> VKDTYTDRLDDWNGIIAGNQYYDSKNDQMAKLNQELEGKVADSLSSISSQADRIYLWEKFSNYKTSANLTATYRKLEEMAKQVTNPSSRYYQDETVVRTVRDSMEWMHKHVYNSEKSIVGNWWDYEIGTPRAINNTLSLMKEYFSDEEIKKYTDVIEKFVPDPEHFRKTTDNPFKALGGNLVDMGRVKVIAGLLRKDDQEISSTIRSIEQVFKLVDQGEGFYQDGSYIDHTNVAYTGAFGNVLIDGLSQLLPVIQKTKNPIDKDKMQTMYHWIDKSFAPLLVNGELMDMSRGRSISRANSEGHVAAVEVLRGIHRIADMSEGETKQRLQSLVKTIVQSDSYYDVFKNLKTYKDISLMQSLLSDAGVASVPRTSYLSAFNKMDKTAMYNAEKGFGFGLSLFSSRTLNYEHMNKENKRGWYTSDGMFYLYNGDLSHYSDGYWPTVNPYKMPGTTETDAKR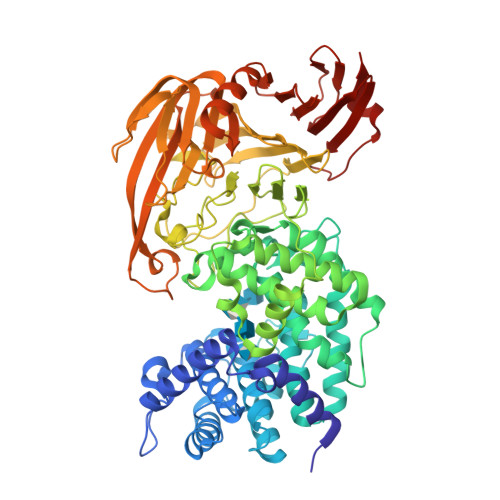ADSDTGKVLPSAFVGTSKLDDANATATMDFTNWNQTLTAHKSWFMLKDKIAFLGSNIQNTSTDTAATTIDQRKLESSNPYKVYVNDKEASLTEQEKDYPETQSVFLESSDSKKNIGYFFFKKSSISMSKALQKGAWKDINEGQSDKEVENEFLTISQAHKQNGDSYGYMLIPNVDRATFNQMIKELESSLIENNETLQSVYDAKQGVWGIVKYDDSVSTISNQFQVLKRGVYTIRKEGDEYKIAYYNPETQESAPDQEVFKKL> MSDSVILRSIKKFGEENDGFESDKSYNNDKKSRLQDEKKGDGVRVGFFQLFRFSSSTDIWLMFVGSLCAFLHGIAQPGVLLIFGTMTDVFIDYDVELQELQIPGKACVNNTIVWTNSSLNQNMTNGTRCGLLNIESEMIKFASYYAGIAVAVLITGYIQICFWVIAAARQIQKMRKFYFRRIMRMEIGWFDCNSVGELNTRFSDDINKINDAIADQMALFIQRMTSTICGFLLGFFRGWKLTLVIISVSPLIGIGAATIGLSVSKFTDYELKAYAKAGVVADEVISSMRTVAAFGGEKREVERYEKNLVFAQRWGIRKGIVMGFFTGFVWCLIFLCYALAFWYGSTLVLDEGEYTPGTLVQIFLSVIVGALNLGNASPCLEAFATGRAAATSIFETIDRK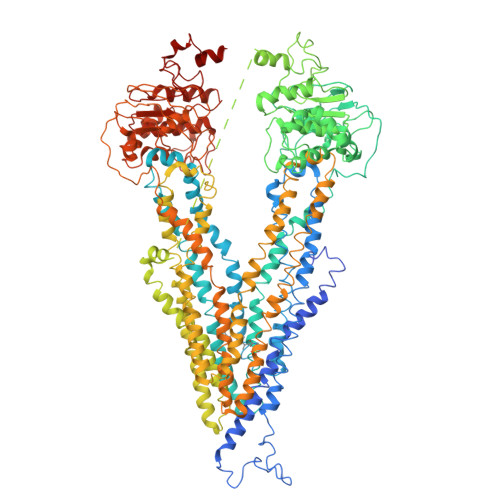PIIDCMSEDGYKLDRIKGEIEFHNVTFHYPSRPEVKILNDLNMVIKPGEMTALVGPSGAGKSTALQLIQRFYDPCEGMVTVDGHDIRSLNIQWLRDQIGIVEQEPVLFSTTIAENIRYGREDATMEDIVQAAKEANAYNFIMDLPQQFDTLVGEGGGQMSGGQKQRVAIARALIRNPKILLLDMATSALDNESEAMVQEVLSKIQHGHTIISVAHRLSTVRAADTIIGFEHGTAVERGTHEELLERKGVYFTLVTLQSQGNQALNEEDIKDATEDDMLARTFSRGSYQDSLRASIRQRSKSQLSYLVHEPPLAVVDHKSTYEEDRKDKDIPVQEEVEPAPVRRILKFSAPEWPYMLVGSVGAAVNGTVTPLYAFLFSQILGTFSIPDKEEQRSQINGVCLLFVAMGCVSLFTQFLQGYAFAKSGELLTKRLRKFGFRAMLGQDIAWFDDLRNSPGALTTRLATDASQVQGAAGSQIGMIVNSFTNVTVAMIIAFSFSWKLSLVILCFFPFLALSGATQTRMLTGFASRDKQALEMVGQITNEALSNIRTVAGIGKERRFIEALETELEKPFKTAIQKANIYGFCFAFAQCIMFIANSASYRYGGYLISNEGLHFSYVFRVISAVVLSATALGRAFSYTPSYAKAKISAARFFQLLDRQPPISVYNTAGEKWDNFQGKIDFVDCKFTYPSRPDSQVLNGLSVSISPGQTLAFVGSSGCGKSTSIQLLERFYDPDQGKVMIDGHDSKKVNVQFLRSNIGIVSQEPVLFACSIMDNIKYGDNTKEIPMERVIAAAKQAQLHDFVMSLPEKYETNVGSQGSQLSRGEKQRIAIARAIVRDPKILLLDEATSALDTESEKTVQVALDKAREGRTCIVIAHRLSTIQNADIIAVMAQGVVIEKGTHEELMAQKGAYYKLVTTGSPIS One mechanism by which phages and other mobile genetic elements are able to overcome the CRISPR-Cas system is through the expression of anti-CRISPR proteins. We previously reported that gene 34 from Pseudomonas phage JBD5, which encodes the protein AcrE1, shows anti-CRISPR activity against the type I-E system of P. aeruginosa strain SMC4386 (4). We show that AcrE1 binds to the CRISPR-associated helicase/nuclease Cas3 and that the C-terminal region of the anti-CRISPR protein is important for its inhibitory activity. In summary, these experiments demonstrate that AcrE1 functions by blocking the activity of Cas3 without inhibiting the DNA-binding activity of Cascade.

Here, we report the 2.5-Å-resolution crystal structure of anti-CRISPR protein AcrE1, which inhibits the type I-E CRISPR-Cas system of P. aeruginosa. (a) Crystal structure of the C-terminal 6×His-tagged AcrE1 solved by Br-SAD reveals a predominantly helical dimeric protein. AcrE1 displays an elongated dimeric structure. Each monomer is predominantly comprised of three helices. Helix 1 (residues 5 to 17) is followed by a tight turn leading into the very long helix 2 (residues 21 to 57). A short turn at the end of helix 2 leads into helix 3 (residues 62 to 80), which terminates close enough to the beginning of helix 1 for a potential H-bond to form between the carbonyl O of Val79 and the amide N of Leu5. Residues 82 to 90 form an antiparallel β-sheet that protrudes at a 90° angle from the end of helix 3. The final 10 residues of AcrE1 are likely disordered, as they were not well defined in the electron density map and could not be modeled into the structure. The large dimeric interface is composed primarily of 18 hydrophobic residues from each monomer that are greater than 97% buried, forming a single hydrophobic core that spans the entire length of the helices. The structure of AcrE1 is not similar to other previously determined anti-CRISPR proteins, and searches using the Dali server did not reveal structural similarity to any other protein.

>MEKKLSDAQVALVAAWRKYPDLRESLEEAASILSLIVFQAETLSDQANELANYIRRQGLEEAEGACRNIDIMRAKWVEVCGEVNQHGIRVYGDAIDRDVDLEHHHHHH[3x]> MEDVEIKPRGYQLRLVDHLTKSNGIVYLPTGSGKTFVAILVLKRFSQDFDKPIESGGKRALFMCNTVELARQQAMAVRRCTNFKVGFYVGEQGVDDWTRGMWSDEIKKNQVLVGTAQVFLDMVTQTYVALSSLSVVIIDECHHGTGHHPFREFMRLFTIANQTKLPRVVGLTGVLIKGNEITNVATKLKELEITYRGNIITVSDTKEMENVMLYATKPTEVMVSFPHQEQVLTVTRLISAEIEKFYVSLDLMNIGVQPIRRSKSLQCLRDPSKKSFVKQLFNDFLYQMKEYGIYAASIAIISLIVEFDIKRRQAETLSVKLMHRTALTLCEKIRHLLVQKLQDMTYDDDDDNVNTEEVIMNFSTPKVQRFLMSLKVSFADKDPKDICCLVFVERRYTCKCIYGLLLNYIQSTPELRNVLTPQFMVGRNNISPDFESVLERKWQKSAIQQFRDGNANLMICSSVLEEGIDVQACNHVFILDPVKTFNMYVQSKGRARTTEAKFVLFTADKEREKTIQQIYQYRKAHNDIAEYLKDRVLEKTEPELYEIKGHFQDDIDPFTNENGAVLLPNNALAILHRYCQTIPTDAFGFVIPWFHVLQEDERDRIFGVSAKGKHVISINMPVNCMLRDTIYSDPMDNVKTAKISAAFKACKVLYSLGELNERFVPKTLKERVASIADVHFEHWNKYGDSVTATVNKADKSKDRTYKTECPLEFYDALPRVGEICYAYEIFLEPQFESCEYTEHMYLNLQTPRNYAILLRNKLPRLAEMPLFSNQGKLHVRVANAPLEVIIQNSEQLELLHQFHGMVFRDILKIWHPFFVLDRRSKENSYLVVPLILGAGEQKCFDWELMTNFRRLPQSHGSNVQQREQQPAPRPEDFEGKIVTQWYANYDKPMLVTKVHRELTPLSYMEKNQQDKTYYEFTMSKYGNRIGDVVHKDKFMIEVRDLTEQLTFYVHNRGKFNAKSKAKMKVILIPELCFNFNFPGDLWLKLIFLPSILNRMYFLLHAEALRKRFNTYLNLHLLPFNGTDYMPRPLEIDYSLKRNVDPLGNVIPTEDIEEPKSLLEPMPTKSIEASVANLEITEFENPWQKYMEPVDLSRNLLSTYPVELDYYYHFSVGNVCEMNEMDFEDKEYWAKNQFHMPTGNIYGNRTPAKTNANVPALMPSKPTVRGKVKPLLILQKTVSKEHITPAEQGEFLAAITASSAADVFDMERLEILGDSFLKLSATLYLASKYSDWNEGTLTEVKSKLVSNRNLLFCLIDADIPKTLNTIQFTPRYTWLPPGISLPHNVLALWRENPEFAKIIGPHNLRDLALGDEESLVKGNCSDINYNRFVEGCRANGQSFYAGADFSSEVNFCVGLVTIPNKVIADTLEALLGVIVKNYGLQHAFKMLEYFKICRADIDKPLTQLLNLELGGKKMRANVNTTEIDGFLINHYYLEKNLGYTFKDRRYLLQALTHPSYPTNRITGSYQELEFIGDAILDFLISAYIFENNTKMNPGALTDLRSALVNNTTLACICVRHRLHFFILAENAKLSEI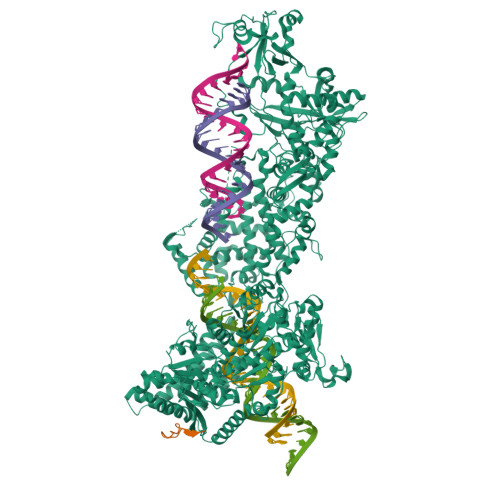ISKFVNFQESQGHRVTNYVRILLEEADVQPTPLDLDDELDMTELPHANKCISQEAEKGVPPKGEFNMSTNVDVPKALGDVLEALIAAVYLDCRDLQRTWEVIFNLFEPELQEFTRKVPINHIRQLVEHKHAKPVFSSPIVEGETVMVSCQFTCMEKTIKVYGFGSNKDQAKLSAAKHALQQLSKCDA;> MDQENFHGSSLPQQLQNLHIQPQQASPNPVQTGFAPRRHYNNLVGLGNGNAVSGSPVKGAPLGQRHVKLKKEKISAQVAQLSQPGQLQLSDVGDPALAGGSGLQGGVGLMGVILPSDEALKFVSETDANGLAMKTPVSILQELLSRRGITPGYELVQIEGAIHEPTFRFRVSFKDKDTPFTAMGAGRSKKEAKHAAARALIDKLIGAQLPESPSSSAGPSVTGLTVAGSGGDGNANATGGGDASDKTVGNPIGWLQEMCMQRRWPPPSYETETEVGLPHERLFTIACSILNYREMGKGKSKKIAKRLAAHRMWMRLQETPIDSGKISDSICGELEGEVSIIQDIDRYEQVSKDFEFIKI>IGSDRVKRGMAEMQKGGVIMDVVNAEQARIAEEAGAVAVMALERVPSDIRAAGGVARMANPKIVEEVMNAVSIPVMAKARIGHITEARVLEAMGVDYIDESEVLTPADEEYHLRKDQFTVPFVCGCRNLGEAARRIGEGAAMLRTKGEPGTGNIVEAVRHMRQVNSEVSRLTVMNDDEIMTFAKDIGAPYEILKQIKDNGRLPVVNFAAGGVATPQDAALMMELGADGVFVGSGIFKSEDPEKFAKAIVQATTHYQDYELIGRLASELGTAMKG[8x]

Here, we investigated the biochemical, structural, and dynamic properties of the enzyme complex responsible for vitamin B6 (pyridoxal 5-phosphate, PLP) biosynthesis in S. aureus, which comprises enzymes SaPdx1 and SaPdx2. A multimeric assembly of two enzymes, Pdx1 and Pdx2, synthesizes pyridoxal 5-phosphate (PLP), the active form of vitamin B6, as well as its vitamers. Pdx2 has glutaminase activity, converting L-glutamine into L-glutamate and an ammonia molecule. The latter is delivered to Pdx1, which synthesizes PLP using ammonia, ribose 5-phosphate (R5P), and glyceraldehyde 3-phosphate (G3P).

Interestingly, independent crystal structures were obtained from crystals with different space groups. However, all the structures revealed the same quaternary arrangement and structural features. The dodecamer forms a cylindrical quaternary structure with an opening diameter of approximately 52 Å and a lateral height of approximately 84 Å. Each monomer is folded as a slightly distorted eight-stranded TIM-barrel with the top of the barrel pointing toward the internal aperture of the cylindrical quaternary structure.> HMRQTIRHSTREKDRGPTKATTTKLVYQIFDTFFAEQIEKDDREDKENAFKRRRCGVCEVCQQPECGKCKACKDMVKFGGSGRSKQACQERRCPNMAMKEADDDEEVDDNIPEMPSPKKMHQGKKKKQNKNRISWVGEAVKTDGKKSYYKKVCIDAETLEVGDCVSVIPDDSSKPLYLARVTALWEDSSNGQMFHAHWFCAGTDTVLGATSDPLELFLVDECEDMQLSYIHSKVKVIYKAPSENWAMEGGMDPESLLEGDDGKTYFYQLWYDQDYARFESPPKTQPTEDNKFKFCVSCAR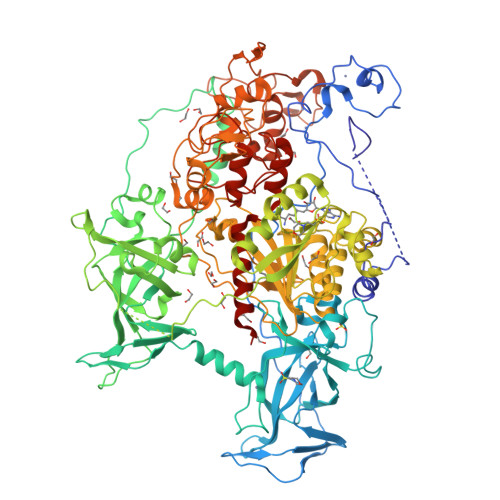LAEMRQKEIPRVLEQLEDLDSRVLYYSATKNGILYRVGDGVYLPPEAFTFNIKLSSPVKRPRKEPVDEDLYPEHYRKYSDYIKGSNLDAPEPYRIGRIKEIFCPKKSNGRPNETDIKIRVNKFYRPENTHKSTPASYHADINLLYWSDEEAVVDFKAVQGRCTVEYGEDLPECVQVYSMGGPNRFYFLEAYNAKSKSFEDPPNHARSPGNKGKGKGKGKGKPKSQACEPSEPEIEIKLPKLRTLDVFSGCGGLSEGFHQAGISDTLWAIEMWDPAAQAFRLNNPGSTVFTEDCNILLKLVMAGETTNSRGQRLPQKGDVEMLCGGPPCQGFSGMNRFNSRTYSKFKNSLVVSFLSYCDYYRPRFFLLENVRNFVSFKRSMVLKLTLRCLVRMGYQCTFGVLQAGQYGVAQTRRRAIILAAAPGEKLPLFPEPLHVFAPRACQLSVVVDDKKFVSNITRLSSGPFRTITVRDTMSDLPEVRNGASALEISYNGEPQSWFQRQLRGAQYQPILRDHICKDMSALVAARMRHIPLAPGSDWRDLPNIEVRLSDGTMARKLRYTHHDRKNGRSSSGALRGVCSCVEAGKACDPAARQFNTLIPWCLPHTGNRHNHWAGLYGRLEWDGFFSTTVTNPEPMGKQGRVLHPEQHRVVSVRECARSQGFPDTYRLFGNILDKHRQVGNAVPPPLAKAIGLEIKLCMLAKA>[4x]QRGLTIWLTGLSASGKSTLAVELEHQLVRDRRVHAYRLDGDNIRFGLNKDLGFSEADRNENIRRIAEVAKLFADSNSIAITSFISPYRKDRDTARQLHEVATPGEETGLP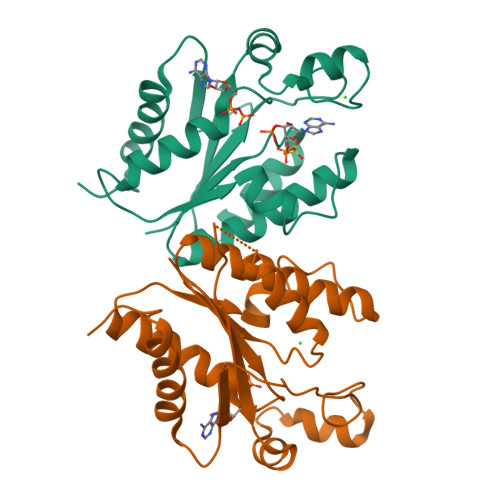FVEVYVDVPVEVAEQRDPKGLYKKAREGVIKEFTGISAPYEAPANPEVHVKNYELPVQDAVKQIIDYLDTKGYLPAKKELEHHHHHH> ADKELKFLVVDDFSTMRRIVRNLLKELGFNNVEEAEDGVDALNKLQAGGYGFVISDWNMPNMDGLELLKT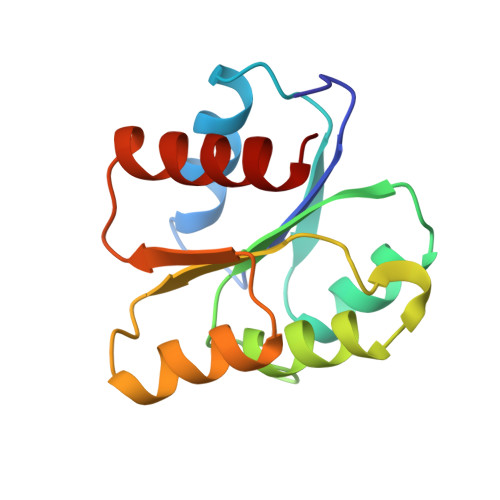IRADGAMSALPVLMVTAEAKKENIIAAAQAGASGYVVKPFTAATLEEKLNKIFEKLGM> NTYQFQNMIQCTVPKRSWRDFADYGCYCGRGGSGTPIDDLDSCCQVHDNCYNSAREQGGCRPKQKTYTYQCKAGGLSCSGANNSCAATTCDCDRLAAICFAGAPYNDNNYNIDLKARCQ;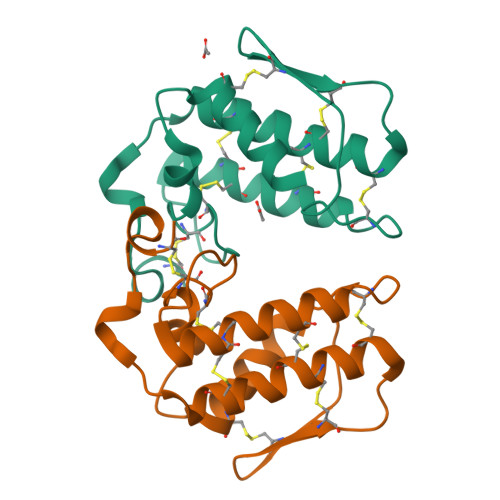> NTWQFKNMISCTVPSRSWWDFADYGCYCGRGGSGTPSDDLDRCCQTHDNCYNEAEKISGCNPRFRTYSYACTAGTLTCTGRNNACAASVCDCDRNAAICFAGAPYNDSNYNIDLQARCN>[4x]MIVSMIAALANNRVIGLDNKMPWHLPAELQLFKRATLGKPIVMGRNTFESIGRPLP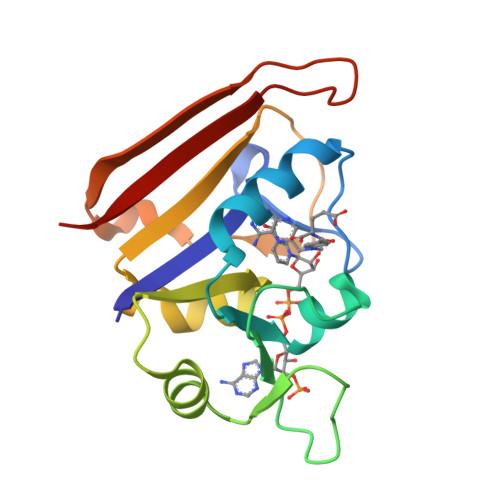GRLNIVLSRQTDYQPEGVTVVATLEDAVVAAGDVEELMIIGGATIYNQCLAAADRLYLTHIELTTEGDTWFPDYEQYNWQEIEHESYAADDKNPHNYRFSLLERVK> PEQ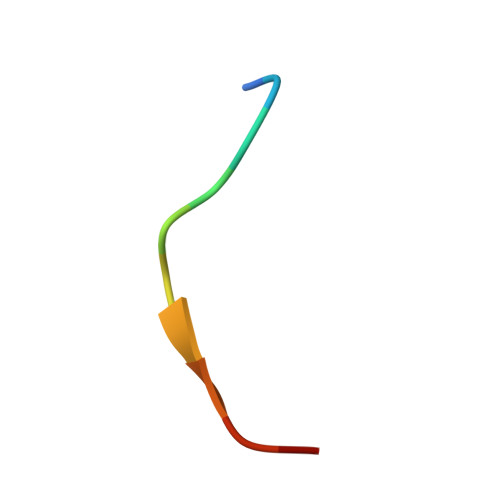DCAVTSGE>MTELSPTALDPTELRSSLDKPFGTNRVIADDAMMADSITPAQYRYHHGSRVRPVNWNNIVDDKDLDVWNRLIANFWLPEKVPLSNDIPSWRSLTDLERKTTTRVFTGLTLLDTSQATIGELCQIEHARTEHEQAIYTNIAFMQSIHARSYSSIFSTLCSSEEIDEAYRWAVGNDVLQQRVTTVLCEYESEDPLKRKIAATMLSSLLLYAGFYLPLYFASRGKMMNTADMIRLILRDKAIHGYYSGYKFQRGLELRSENDKKNLEKFTMNLLDTLYDLEVEYSGQIYEGFDFHDDVFDFVRYNANKALMNLGYPAKYSEEETHVSPEILAALSPAADENHDFFSGSGSSYIMGKSVETDDDDWDFLEHHHHHH[4x]

Class I ribonucleotide reductases (RNRs) convert ribonucleotides into deoxyribonucleotides under oxic conditions. The R2 subunit provides a radical required for catalysis conducted by the R1 subunit. The discovery of a metal-free R2 defined the new RNR subclass Ie. In R2e, three of the otherwise strictly conserved metal-binding glutamates in the active site are substituted.

The second crystal structure we solved was from R2 protein coexpressed with R1, NrdI and NrdH, hereafter called BvR2eQSK-DOPA. Crystals belong to the same space group with similar unit cell dimensions and resolution. The two structures are similar overall with an Cα root-mean-square deviation (RMSD) value of 0.16 Å. The conserved tyrosine close to the active site shows an additional density, corresponding to a modification to a DOPA. Composite omit maps confirmed that the tyrosine is modified between structures. Overlaying both structures shows no further structural reorganization; all other active site residues are in the same position. The conformation of the active site residues DOPA150, D112 and K237 aligns best with the radical-lost ground state of MfR2e and differs from the radical state, suggesting that we observe an inactive state of the protein in our structures. However, the hydrogen bonding network and water structure in the active site between the VPK and QSK versions of R2 are clearly different due to the bulkier Q and S compared to V and P. This will likely contribute to the differences in activity between R2eVPK and R2eQSK. The in vitro activity of RNRQSK is therefore dependent on the presence of DOPA in R2 and reduced NrdI in an aerobic environment.(2~{S})-2-acetamido-~{N}-(3-bromanylprop-2-ynyl)butanediamide | C9 H12 Br 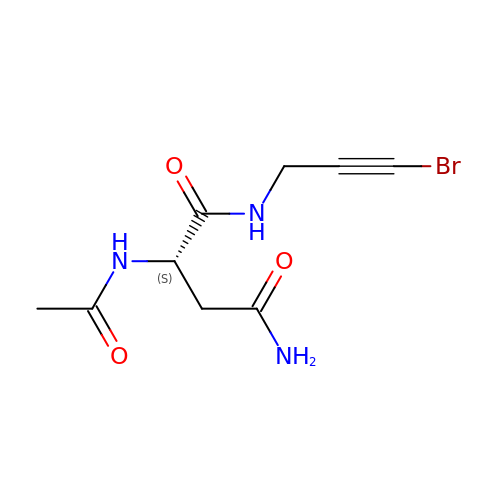N3 O3 | JMTFRQZEUVQLRL-ZETCQYMHSA-N>[2x]MAHHHHHHMSRMAEQQLYINGGYTSATSGRTFETINPATGEVLATVQAAGREDVDRAVESAQRGQKIWAAMTAMERSRILRRAVDLLRQRNDELARLETLDTGKPLSETAAVDIVTGADVLEYYAGLIPALEGSQIPLRDSSFVYTRREPLGVVAGIGAWNYPIQIALWKSAPALAAGNAMIFKPSEVTPLT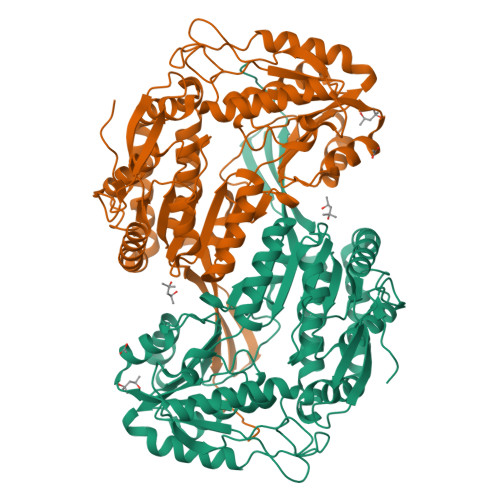ALKLAEIYSEAGLPDGVFNVLPGIGAETGQYLTEHPDIAKISFTGGVASGKKVMANSAASSLKEVTMELGGKSPLIIADDADLDLAADIAMMANFYSSGQVCTNGTRVFVPAKQKAEFEHKILERVARIRPGDLFADDTNFGPLVSFPHRDNVLRYIESGKREGARLLCGGEALKGDGFDNGSWVAPTVFTDCSDEMTIVREEIFGPVMSILSYADEAEVIRRANATEYGLAAGVVTPNLNRAHRIIHQLEAGICWINSWGESPAEMPVGGYKHSGIGRENGVMTLQSYTQVKSIQVEMGKFQSIF> RDERYPTQSPMPLTVACASPELASGKVWIR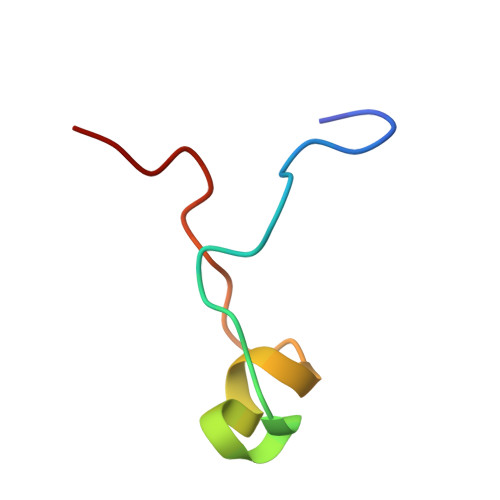YPIVR>MIQTERAVQQVLEWGRSLTGFADEHAVEAVRGGQYILQRIHPSLRGTSARTGRDPQDETLIVTFYRELALLFWLDDCNDLGLISPEQLAAVEQALGQGVPCALPGFEGCAVLRASLATLAYDRRDYAQLLDDTRCYSAALRAGHAQAVAAERWSYAEYLHNGIDSIAYANVFCCLSLLWGLDMATLRARPAFRQVLRLISAIGRLQNDLHGCDKDRSAGEADNAVILLLQRYPAMPVVEFLNDELAGHTRMLHRVMAEERFPAPWG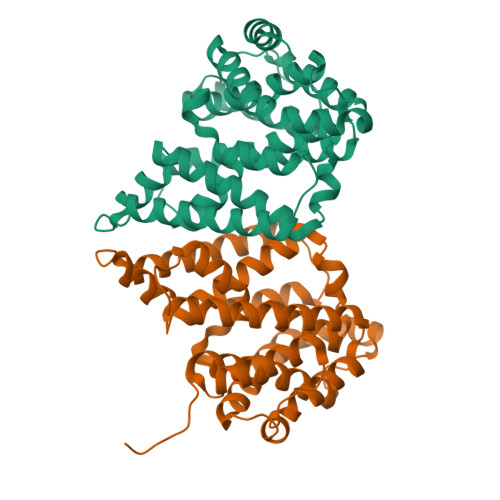PLIEAMAAIRVQYYRTSTSRYRSDAVRGGQRAPA[2x]>[2x]GSHMSGEDAEVRAVSEDVSNGSSGSPSPGDTLPWNLGKTQRSRRSGGGAGSNGSVLDPAERAVIRIADERDRVQKKTFTKWVNKHLIKAQRHISDLYEDLRDGHNLISLLEVLSGDSLPREKGRMRFHKLQNVQIALDYLRHRQVKLVNIRNDDIADGNPKLTLGLIWTIILHFQISDIQVSGQSEDMTAKEKLLLWSQRMVEGYQGLRCDNFTSSWRDGRLFNAIIHRHKPLLIDMNKVYRQTNLENLDQAFSVAERDLGVTRLLDPEDVDVPQPDEKSIITYVSSLYDAMPRVP;>GSHDLGAPQNPNAKAAGSRKIHFNWLPPSGKPMGYRVKYWIQGDSESEAHLLDSKVPSVELTNLYPYCDYEMKVCAYGAQGEGPYSSLVSCRTHQEVPSEPGR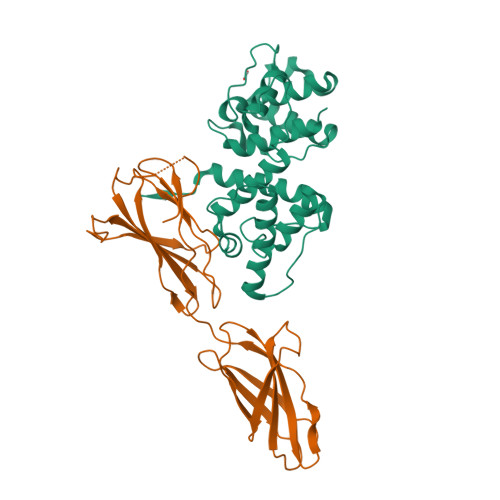LAFNVVSSTVTQLSWAEPAETNGEITAYEVCYGLVNDDNRPIGPMKKVLVDNPKNRMLLIENLRESQPYRYTVKARNGAGWGPEREAIINLATQPKRPMSIPIIPDIPIVDAQSGEDYDSFLMYSDDVLRSPSGSQRPSVSDDTE[3x]4-[3-amino-4-(4-hydroxyphenyl)-1H-pyrazol-5-yl]benzene-1,3-diol 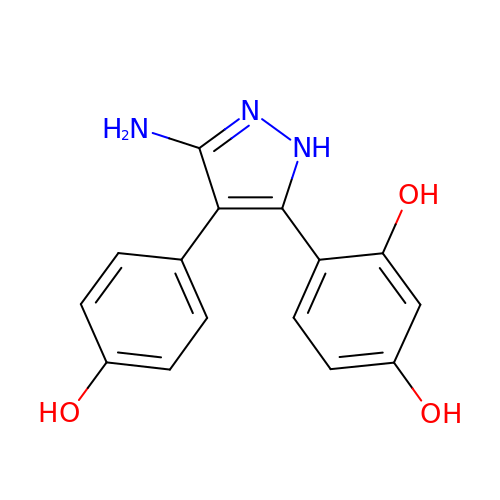| C15 H13 N3 O3 | QJXCNANYVSBOBZ-UHFFFAOYSA-N> MASMTGGQQMGRGSMIFSVDKVRADFPVLSREVNGLPL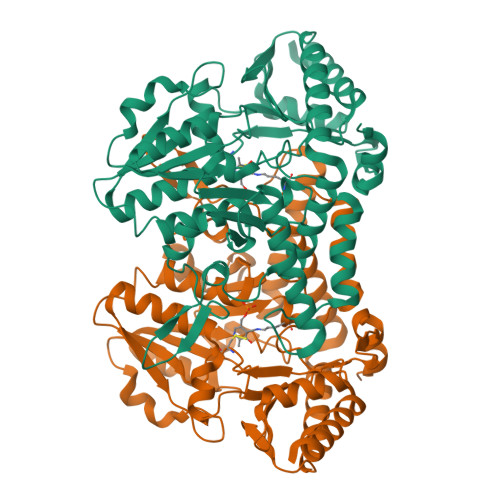AYLDSAASAQKPSQVIDAEAEFYRHGYAAVHRGIHTLSAQATEKMENVRKRASLFINARSAEELVFVRGTTEGINLVANSWGNSNVRAGDNIIISQMEHHANIVPWQMLCARVGAELRVIPLNPDGTLQLETLPTLFDEKTRLLAITHVSNVLGTENPLAEMITLAHQHGAKVLVDGAQAVMHHPVDVQALDCDFYVFSGHKLYGPTGIGILYVKEALLQEMPPWEGGGSMIATVSLSEGTTWTKAPWRFEAGTPNTGGIIGLGAALEYVSALGLNNIAEYEQNLMHYALSQLESVPDLTLYGPQNRLGVIAFNLGKHHAYDVGSFLDNYGIAVRTGHHCAMPLMAYYNVPAMCRASLAMYNTHEEVDRLVTGLQRIHRLLG>[2x]GSGMLNRVEDILHEL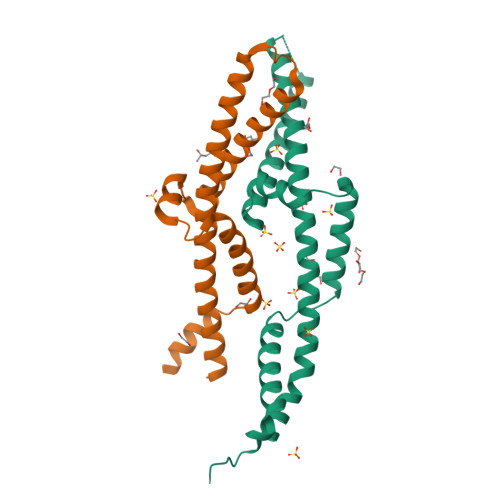EGQVEPLKIQASIAKDYLEKKKELEHVEIALTAYDIEELHGKWSTLKEKVQMAKESGGSGGSTLLKDEEVKLGRMEVELDNLLQYLREEYSLSFEGAKEKYQLETDPEEARKRVKLIKLAIEELGTVNLGSIDEFERVNERYKFLSEQKEDL>[2x]MANTRVIELFDEFTDLIRDFIVRHEITTPEY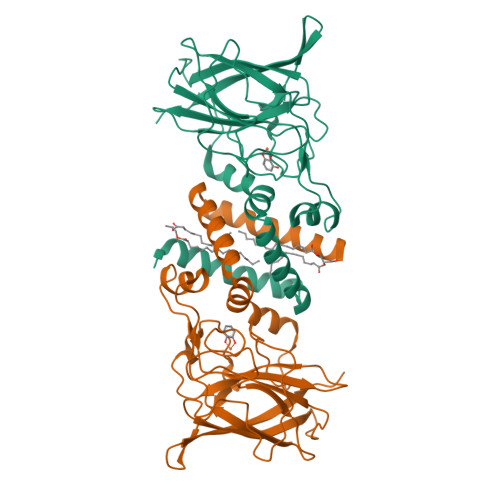ETIMQYMISVGEAGEWPLWLDAFFETTVDSVSYGKGNWTSSAIQGPFFKEGAPLLTGKPATLPMRADEPGDRMRFTGSVRDTSGTPITGAVIDVWHSTNDGNYSFFSPALPDQYLLRGRVVPAEDGSIEFHSIRPVPYEIPKAGPTGQLMNSYLGRHSWRPAHIHIRITADGYRPLITQLYFEGDPYLDSDSCSAVKSELVLPVNKIDIDGETWQLVDFNFILQHN> MSEAPKKRWYVVQAFSGFEGRVATSLREHIKLHNMEDLFGEVMVPTEEVVEIRGGQRRKSERKFFPGYVLVQMVM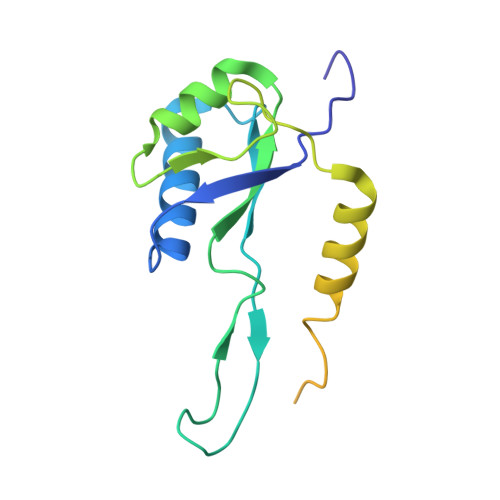NDASWHLVRSVPRVMGFIGGTSDRPAPISDKEVDAIMNRLQQVGDKPRPKTLFEPGEMVRVNDGPFADFNGVVEEVDYEKSRLKVSVSIFGRATPVELDFSQVEKA> VIDRLVVQTSSGPVRGRSVTVQGREVHVYTGIPYAKPPVEDLRFRKPVPAEPWHGVLDATGLSATCVQERYEYFPGFSGEEIWNPNTNVSEDCLYINVWAPAKARLRHGRGANGGEHPNGKQADTDHLIHNGNPQNTTNGLPILIWIYGGGFMTGSATLDIYNADIMAAVGNVIVASFQYRVGAFGFLHLAPEMPSEFAEEAPGNVGLWDQALAIRWLKDNAHAFGGNPEWMTLFGESAGSSSVNAQLMSPVTRGLVKRGMMQSGTMNAPWSHMTSEKAVEIGKALINDCNCNASMLKTNPAHVMSCMRSVDAKTISVQQWNSYSGILSFPSAPTIDGAFLPADPMTLMKTADLKDYDILMGNVRDEGTYFLLYDFIDYFDKDDATALPRDKYLEIMNNIFGKATQAEREAIIFQYTSWEGNPGYQNQQQIGRAVGDHFFTCPTNEYAQALAERGASVHYYYFTHRTSTSLWGEWMGVLHGDEIEYFFGQPLNNSLQYRPVERELGKRMLSAVIEFAKTGNPAQDGEEWPNFSKEDPVYYIFSTDD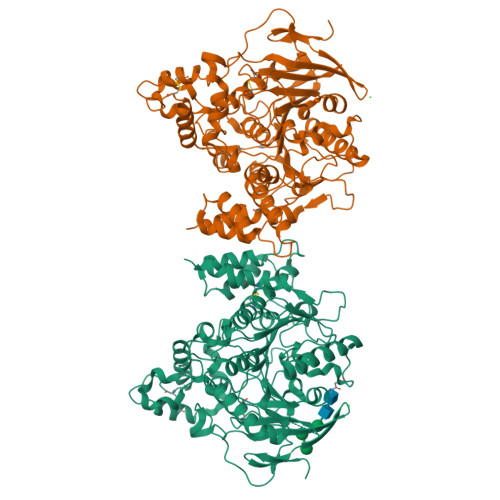KIEKLARGPLAARCSFWNDYLPKVRSWAGTCDGDS1-AZEPAN-1-YL-2-PHENYL-2-(4-THIOXO-1,4-DIHYDRO-PYRAZOLO[3,4-D]PYRIMIDIN-5-YL)ETHANONE ADDUCT | C40 H44 N12 O15 P2 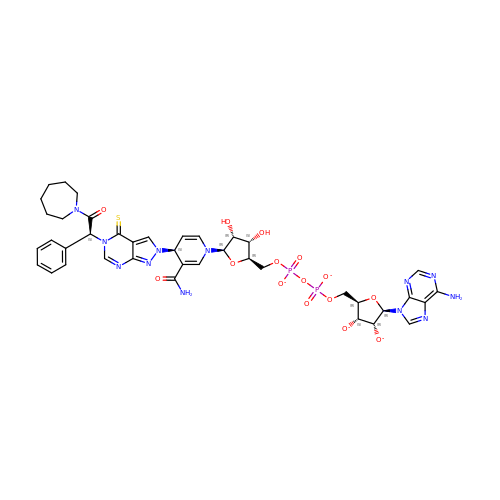S | XHBACRZQFHLVAV-LFFSAXSQSA-L>GSGRGLGPLQIWQTDFTLEPRMAPRSWLAVTVDTASSAIVVTQHGRVTSVAAQHHWATAIAVLGRPKAIKTDNGSCFTSKSTREWLARWGIAHTTG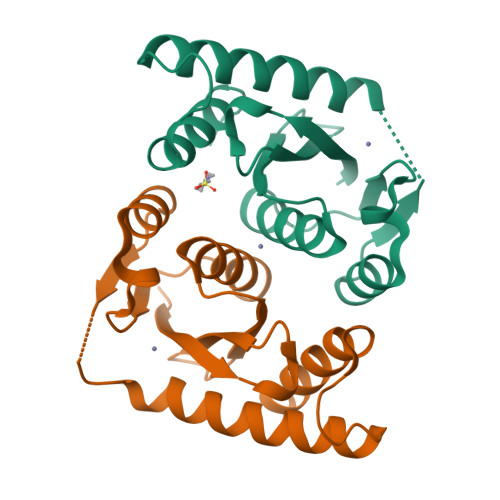IPGNSQGQAMVERANRLLKDKIRVLAEGDGFMKRIPASKQGELLAKAMYALNHF[2x]>[2x]HGFVSGIVADGKYYGGYLVNQYPYMSNPPDTIAWSTTATDLGFVDGTGYQSPDIICHRDAKNGKLTATVAAGSQIEFQWTTWP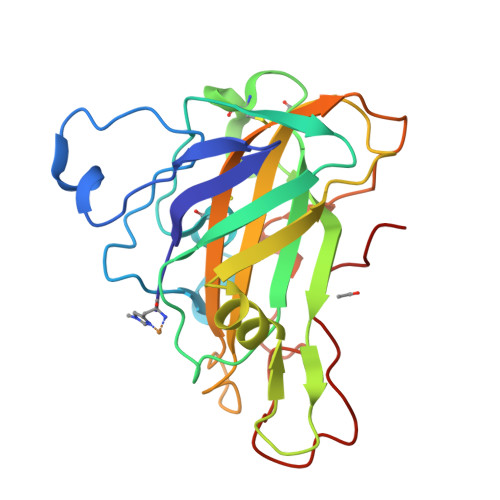ESHHGPVITYLAPCNGDCATVDKTTLKFVKIAAQGLIDGSNPPGVWASDELIANNNTWTVTIPASYAPGNYVLRHEIIALHSAGNLNGAQNYPQCFNIQITGGGSAQGSGTAGTSLYKNTDPGIKFDIYSDLSGGYPIPGPALFNA>DWVIPPISCPENEKGEFPKNLVQIKSNRDKETKVFYSITGQGADKPPVGVFIIERETGWLKVTQPLDREAIAKYILYSHAVSSNGEAVEDPMEIVITVTDQNDNRPEFTQEVFEGSVAEGAVPGTSVMKVSATDADDDVNTYNAAIAYTIVSQDPELPHKNMFTVNRDTGVISVLTSGLDRESYPTYTLVVQAADLQGEGLSTTAKAVITVKDINDNAPVFNPSTYQGQVPENEVNARIATLKVTDDDAPNTPAWKAVYTVVNDPDQQFVVVTDPTTNDGILKTAKGLDFEAKQQYILHVRVENEEPFEGSLVPSTATVTVDVVDVNEAPIFMPAERRVEVPEDFGVGQEITSYTAREPDTFMDQKITYRIWRDTANWLEINPETGAIFTRAEMDREDAEHVKNSTYVALIIATDDGSPIATGTGTLLLVLLDVN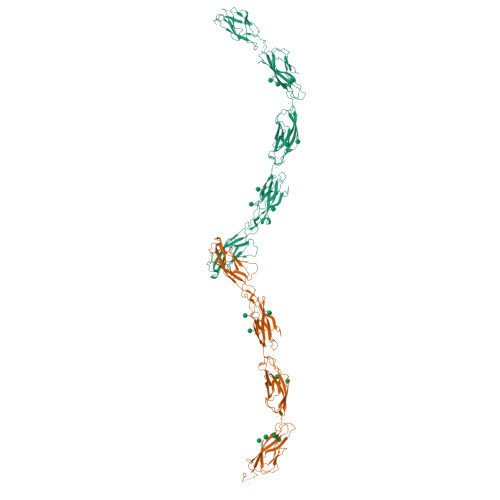DNAPIPEPRNMQFCQRNPQPHIITILDPDLPPNTSPFTAELTHGASVNWTIEYNDAAQESLILQPRKDLEIGEYKIHLKLADNQNKDQVTTLDVHVCDCEGTVNNCMKAHHHHHH[2x]>MTMEQFLTSLDMIRSGCAPKFKLKTEDLDRLRVGDF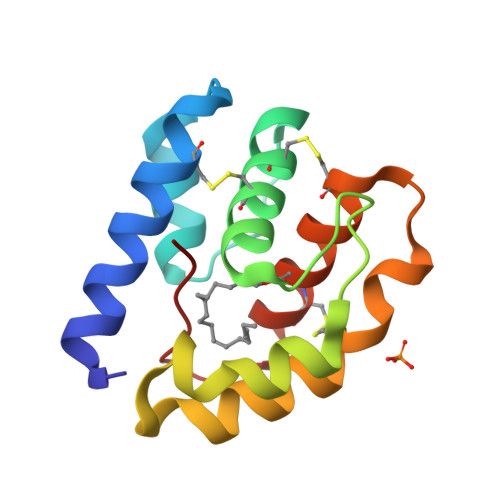NFPPSQDLMCYTKCVSLMAGTVNKKGEFNAPKALAQLPHLVPPEMMEMSRKSVEACRDTHKQFKESCERVYQTAKCFSENADGQFMWP[2x]>[2x]MIQQTGYSKKVMEHFMNPRNVGVIDDPDGYGKVGNPVCGDLMEIFI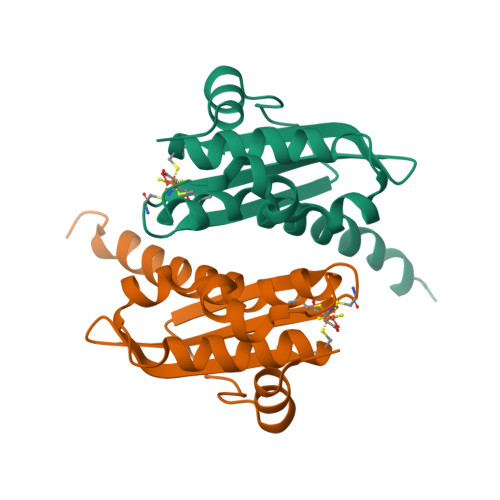KVGDEKIEDIKFRTFGCGAAIATSSMITEMARGKSLEEAMRITRNDVADALDGLPPQKMHCSNLAADALHAAINDYLSKKQKHLEHHHHHH{[(2S)-3-(2-amino-6-oxo-1,6-dihydro-9H-purin-9-yl)propane-1,2-diyl]bis(oxyethane-2,1-diyl)}bis(phosphonic 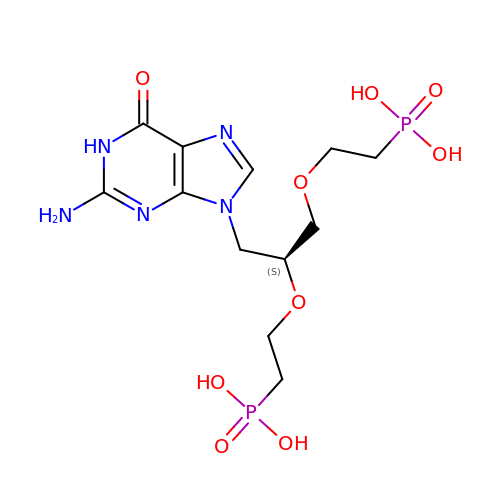acid) | C12 H21 N5 O9 P2 | KFMQQVHVLQIQPE-QMMMGPOBSA-N> HHHHHHDITFRNIRFRYKPDSPV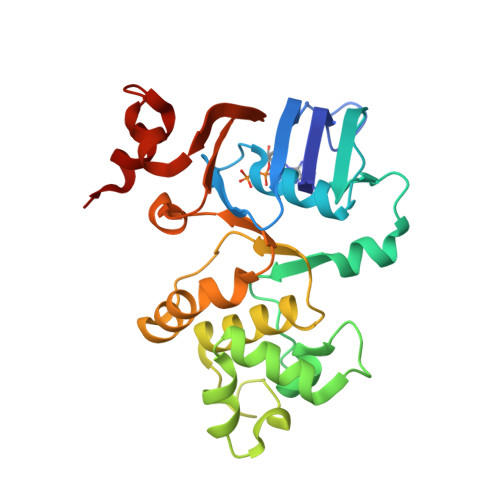ILDNINLSIKQGEVIGIVGRSGSGKSTLTKLIQRFYIPENGQVLIDGHDLALADPNWLRRQVGVVLQDNVLLNRSIIDNISLANPGMSVEKVIYAAKLAGAHDFISELREGYNTIVGEQGAGLSGGQRQRIAIARALVNNPKILIFDQATSALDYESEHVIMRNMHKICKGRTVIIIAHRLSTVKNADRIIVMEKGKIVEQGKHKELLSEPESLYSYLYQLQSD>HMSVNKVTCLVCRKGDNDEFLLLCDGCDRGCHIYCHRPKMEAVPEGDWFCTVCLAQQV[4x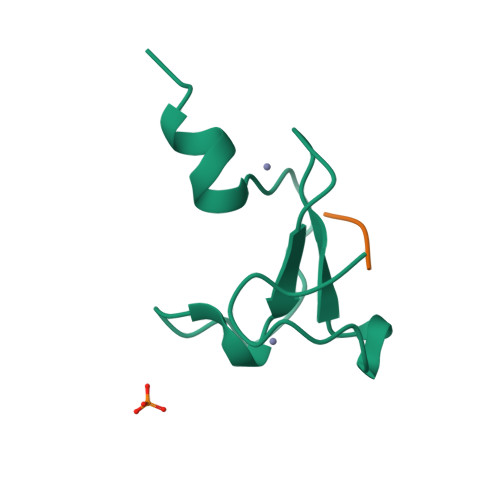]> SVVIPTHAQKDMVGRGHAWLKGDNIRDHVTRVEGWMWKNKLLTVAVVALAWLMLDSWMARVTVILLAL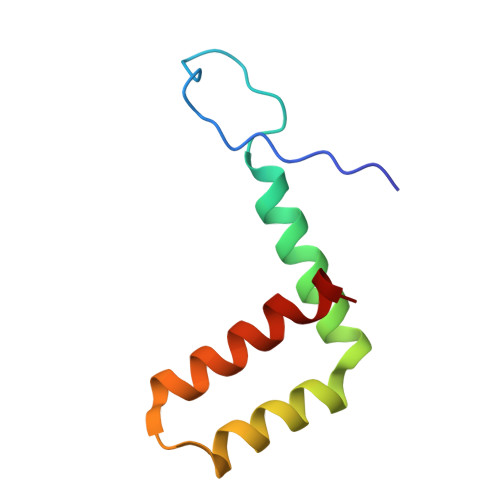SLGPVYA> MHMLRIAKEALTFDDVLLVPAHSTVLPNTADLRTRLTKNIALNIPMVSASMDTVTEARLAIALAQEGGIGFIHKNMSIEQQAAQVHQVKIFEAGVVTHPVTVRPEQTIADVMELTHYHGFAGFPVVTENNELVGIITGRDVRFVTDLTKSVAAVMTPKERLATVKEGATGAEVQEKMHKARVEKILVVNDEFQLKGMITAKDFHKAESKPNACKDEQGRLRVGAAVGAAPGNEERVKALVEAGVDVLLIDSSHGHSEGVLQRIR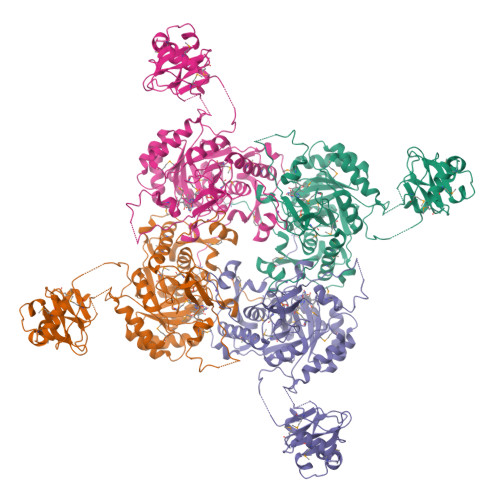ETRAAYPHLEIIGGNVATAEGARALIEAGVSAVKVGIGPGSICTTRIVTGVGVPQITAIADAAGVANEYGIPVIADGGIRFSGDISKAIAAGASCVMVGSMFAGTEEAPGEVILYQGRSYKAYRGMGSLGAMSKGSSDRYFQTDNAADKLVPEGIEGRIAYKGHLKEIIHQQMGGLRSCMGLTGSATVEDLRTKAQFVRISGAGMKESHVHDVQITKEAPNYRLGGENLYFQ>[14x]MIDVSSQRVNVQRPLDALGNSLNSPVIIKLKGDREFRGVLKSFDLHMNLVLN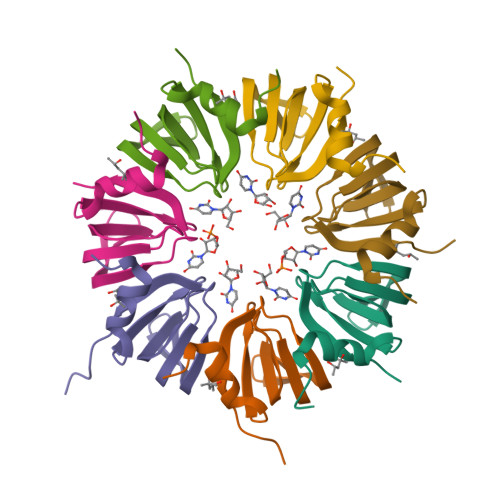DAEELEDGEVTRRLGTVLIRGDNIVYISRGKLAAA> MWELTILHTNDVHSRLEQTSEDSSKCVDASRCMGGVARLFTKVQQIRRAEPNVLLLDAGDQYQGTIWFTVYKGAEVAHFMNALRYDAMALGNHEFDNGVEGLIEPLLKEAKFPILSANIKAKGPLASQISGLYLPYKVLPVGDEVVGIVGYTSKETPFLSNPGTNLVFEDEITALQPEVDKLKTLNVNKIIALGHSGFEMDKLIAQKVRGVDVVVGGHSNTFLYTGNPPSKEVPAGKYPFIVTSDDGRKVPVVQAYAFGKYLGYLKIEFDERGNVISSHGNPILLDSSIPEDPSIKADINKWRIKLDDYSTQELGKTIVYLDGSSQSCRFRECNMGNLICDAMINNNLRHTDEMFWNHVSMCILNGGGIRSPIDERNDGTITWENLAAVLPFGGTFDLVQLK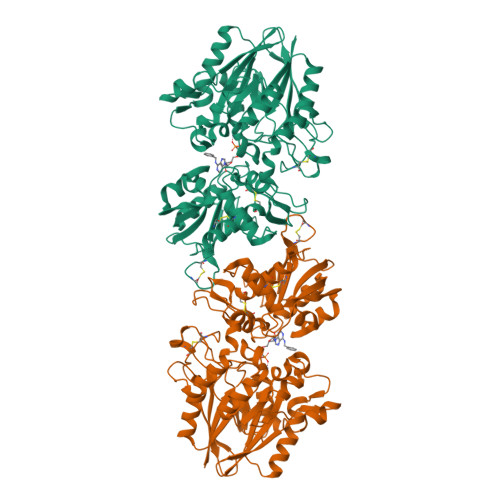GSTLKKAFEHSVHRYGQSTGEFLQVGGIHVVYDLSRKPGDRVVKLDVLCTKCRVPSYDPLKMDEVYKVILPNFLANGGDGFQMIKDELLRHDSGDQDINVVSTYISKMKVIYPAVEGRIKFSLEHHHHHH S-(P-NITROBENZYL)GLUTATHIONE | C17 H22 N4 O8 S 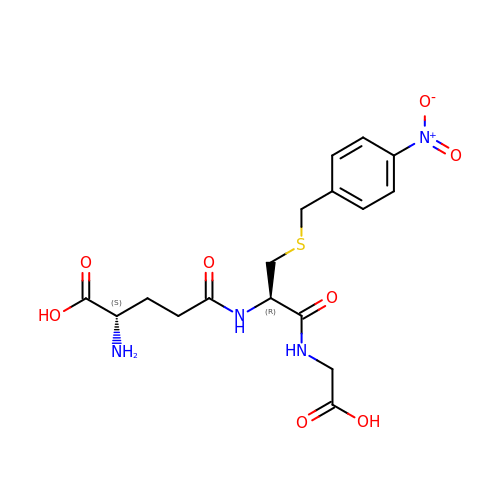| OAWORKDPTSAMBZ-STQMWFEESA-N>MKAHPKEMVPLMGKRVAAPSGNPAVLPEKRPAEITPTKKSAHFFLEIEGFEPNPTVAKTSPPVFSKPMDSNIRQCISGNCDDMDSPQSPQDDVTETPSNPNSPSAQLAKEEQRRKKRRLKKRIFAAVSEGCVEELVELLVELQELCRRRHDEDVPDFLMHKLTASDTGKTCLMKALLNINPNTKEIVRILLAFAEENDILGRFINAEYTEEAYEGQTALNIAIERRQGDIAALLIAAGADVNAHAKGAFFNPKYQHEGFYFGETPLALAACTNQPEIVQLLMEHEQTDITSRDSRGNNILHALVTVAEDFKTQNDFVKRMYDMILLRSGNWELETTRNNDGLTPLQLAAKMGKAEILKYILSREIKEKRLRSLSRKFTDWAYGPVSSSLYDLTNVDTTTDNSVLEITVYNTNIDNRHEMLTLEPLHTLLHMKWKKFAKHMFFLSFCFYFFYNITLTLVSYYRPREEEAIPHPLALTHKMGWLQLLGRMFVLIWAMCISVKEGIAIFLLRPSDLQSILSDAWFHFVFFIQAVLVILSVFLYLFAYKEYLACLVLAMALGWANMLYYTRGFQSMGMYSVMIQKVILHDVLKFLFVYIVFLLGFGVALASLIEKCPKDNKDCSSYGSFSDAVLELFKLTIGLGDLNIQQNSKYPILFLFLLITYVILTFVLLLNMLIALMGETVENVSKESERIWRLQRARTILEFEKMLPEWLRSRFRMGELC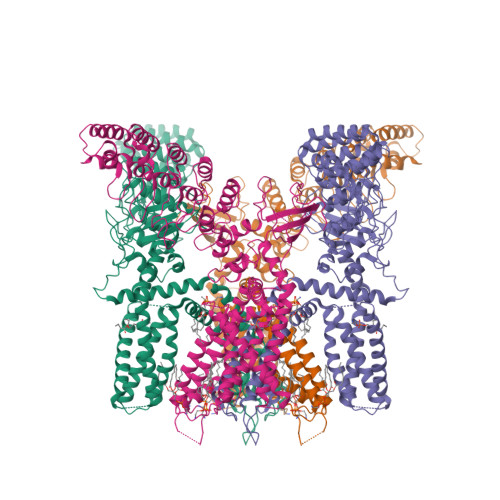KVAEDDFRLCLRINEVKWTEWKTHVSFLNEDPGPVRRTDFNKIQDSSRNNSKTTLNAFEEVEEFPETSV[4x]> GDPHMSLSVAEKSYLYDSLASTPSIRPDGRLPHQFRPIEIFTDFLPSSNGSSRIIASDGSECIVSIKSKVVDHHVENELLQVDVDIAGQRDDALVVETITSLLNKVLKSGSGVDSSKLQLTKKYSFKIFVDVLVISSHSHPVSLISFAIYSALNSTYLPKLISAFDDLEVEELPTFHDYDMVKLDI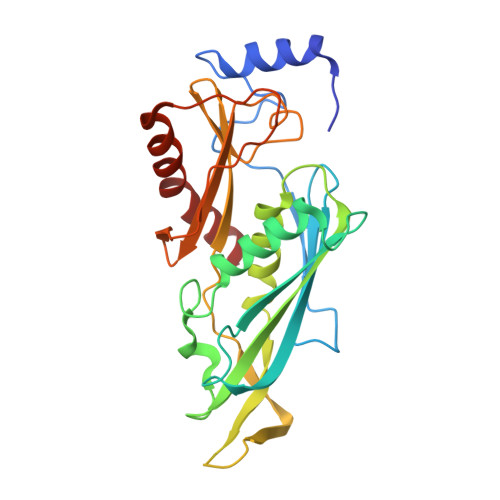NPPLVFILAVVGNNMLLDPAANESEVANNGLIISWSNGKITSPIRSVALNDSNVKSFKPHLLKQGLAMVEKYAPDVVRSLENL>TSEINLRIEPFSSPFATDLAKLQTQIGYKFNNINLLRRAMTHASFSQENNKA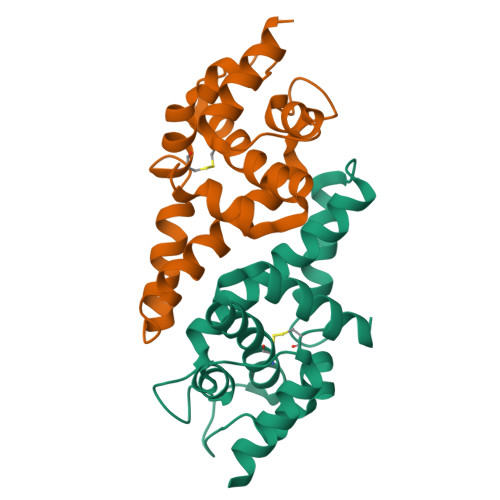LSIFGTHIIETAVSLQFLAKDIDISSKALGRLISEVSNVESSCALDGDRLGLGKIIRVSTKTDASNSAILCTGFRAIFGAIAIDAGTVDEAIKVFWKVHGARAGRLVSMLS[2x]> MRGSHHHHHHGSPYNVMIVDDAAMMRLYIASFIKTLPDFKVVAQAANGQE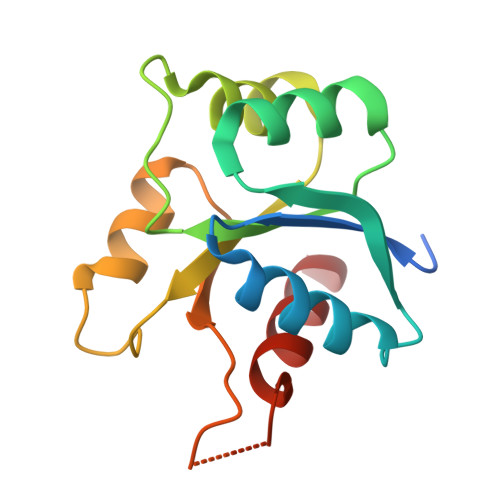ALDKLAAQPNVDLILLDIEMPVMDGMEFLRHAKLKTRAKICMLSSVAVSGSPHAARARELGADGVVAKPSGTVSHDLEEKTGGELARTMRTLMAA>[2x]MDSKDQTMFYNFGDDSIEEDVKKLMKQVYVALEEKG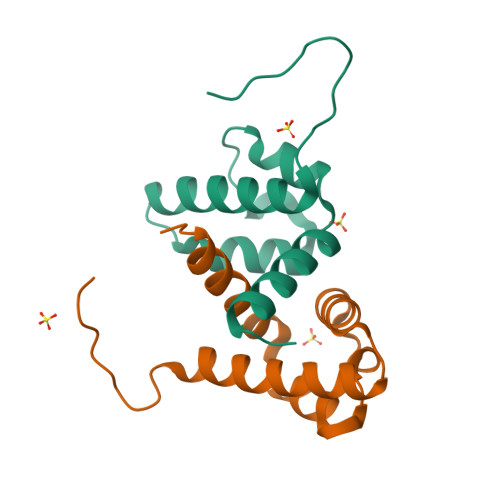YNPVNQIVGYLLSGDPAYIPRHKDARSMIRRLERDEIIEELVKAYLKNNEIGEK> GSDLTVSLIPVSGLKAGKNAPSAKIAKLVVNSTT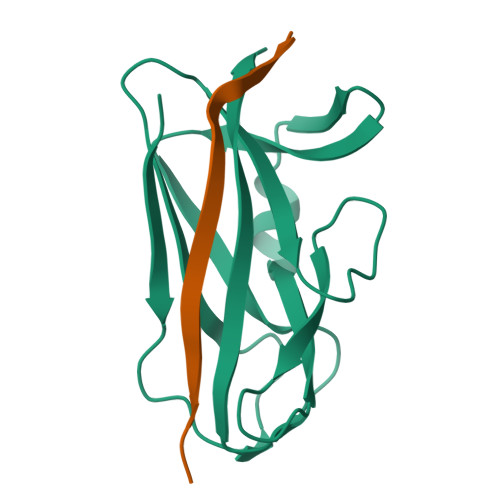LKEFGVRGISNNVVDSTGTAWRVAGKNTGKEIGVGLSSDSLRRSDSTEKWNGVNWMTFNSNDTLDIVLTGPAQNVTADTYPITLDVVGYQP;> GSFLPNSEQQKSVDAVFSSP~{N}-[(1~{S})-1-(3,4-dihydro-2~{H}-1,5-benzodioxepin-7-yl)ethyl]-2-methyl-pyridin-3-amine 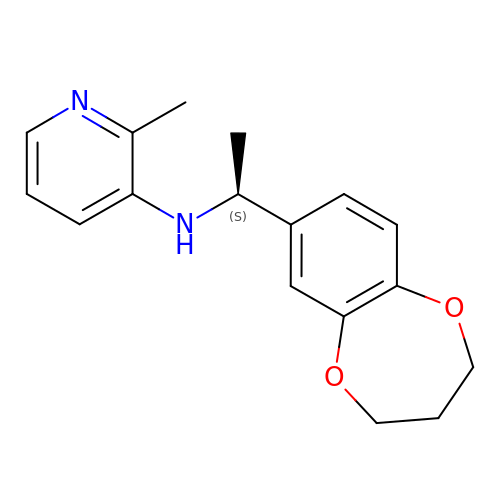| C17 H20 N2 O2 | XKZPCVJIRSIGQB-LBPRGKRZSA-N>[2x]GSLVPRGSPSRSEFTEWRFPKSTCPGRSLQKMLQLNPHRHATAGSQAATIPNREPFISCSQDECRLFTLDHDVSTPGAYDGITWEDRSKRRRLVSFPLGSELTLDNMKVHLSGWSGTACHDGKEWTYATVNGPDNSAVMRLKYGDQIRGSFPSYANNILRTQESECVCIDGKCYIIVIDGPAGGTATPKVLVTREGEVTSEIIVTGRNKMGE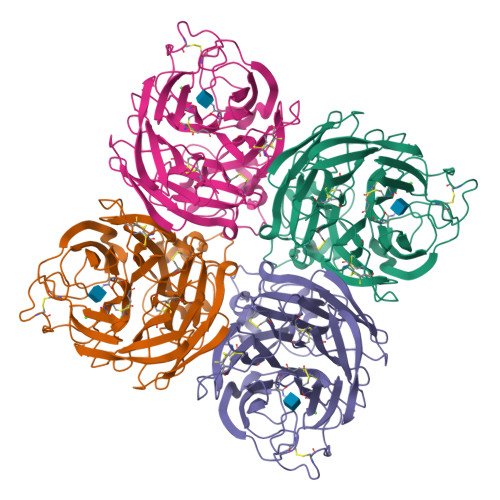ECSCLATNRTWIECLCRDNAFSAKRPIIRIDTVAGTARGYLMCSDTYLDTPRPADGSITGSCETDGTSGGGGVKGAFALSRTTEATTERFYVRTVSSSARSGAVFYKTTDDPTESNNPLTLIGTAVGGAIPMWYSFSFEIPGKVCDQTCIGLEMGLTMGHQLWTSNSVAVYCVIGDNLDWDSTTDVVPADIV> MKLIAESGSTKTEWSLVEGEHLIQRVFTEGLNPFFQTRREISRSIRLGL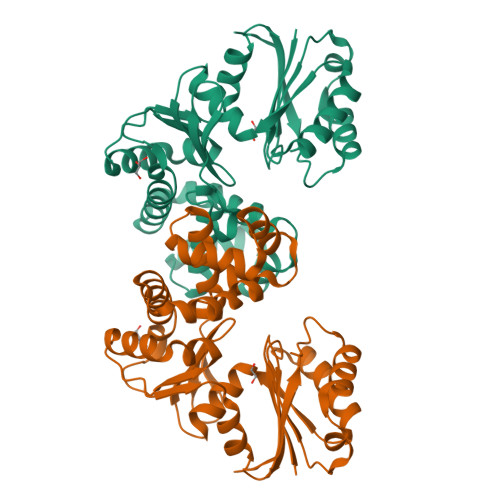PDSFFKRKLEQVFFYGAGCTSAEKKSVVEASLVAQFKTPAYVESDLLAAARGLFQHDSGIACILGTGSNSCFYDGHVIVKNVRAGGYILGDEGSGAALGKQFLSDVLKKLAPQVLIDDFFEKYDLTPHDVMDVVYNRPFPNRFLAEQSCFLADYLRLDYVKGLLLSNLRSFFLRNVMQYDYLNYPIRFVGSVAYNYADLLHQVGKEFGVELSVVEETPMGGLIKYHAFPPDDPES> EITIGVLSLQGDFEPHINHFIKLQIPSLNIIQVRNVHDLGLCDGLVIPGGESTTVRRCCAYENDTLYNALVHFIHVLKKPIWGTCAGCILLSKNVENIKLYSNFGNKFSFGGLDITICRNFYGSQNDSFICSLNIISDSSAFKKDLTAACIRAPYIREILSDEVKVLATFSHESYGPNIIAAVEQNNCLGTVF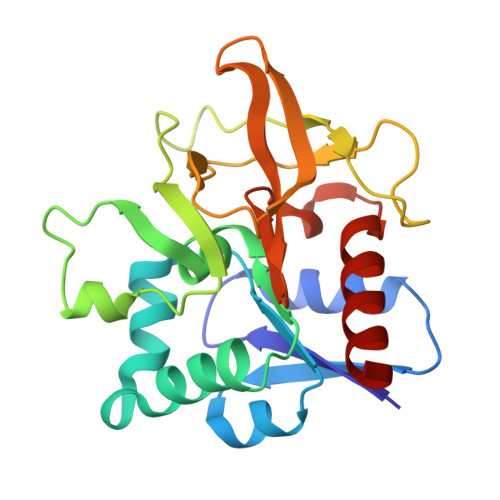NPELLPHTAFQQYFYEKVKNYKYS> MLTQKTKDIVKATAPVLAEHGYDIIKCFYQRMFEAHPELKNVFNMAHQEQGQQQQALARAVYAYAENIEDPNSLMAVLKNIANKHASLGVKPEQYPIVGEHLLAAIKEVLGNAATDDIISAWAQAYGNLADVLMGMESELYERSAEQPGGWKGWRTFVIREKRPESDVITSFILEPADGGPVVNFEPGQYTSVAIDVPALGLQQIRQYSLSDMPNGRSYRI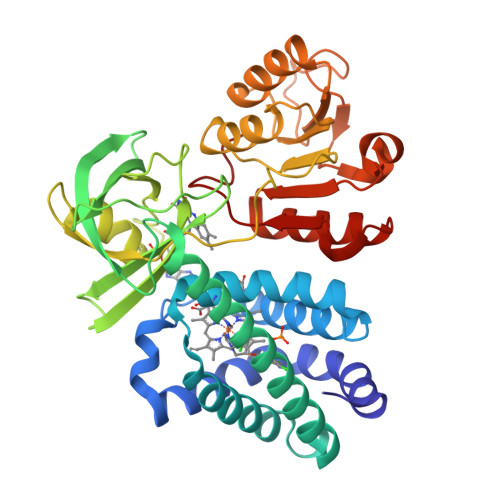SVKREGGGPQPPGYVSNLLHDHVNVGDQVKLAAPYGSFHIDVDAKTPIVLISGGVGLTPMVSMLKVALQAPPRQVVFVHGARNSAVHAMRDRLREAAKTYENLDLFVFYDQPLPEDVQGRDYDYPGLVDVKQIEKSILLPDADYYICGPIPFMRMQHDALKNLGIHEARIHYEVFGPDLFAE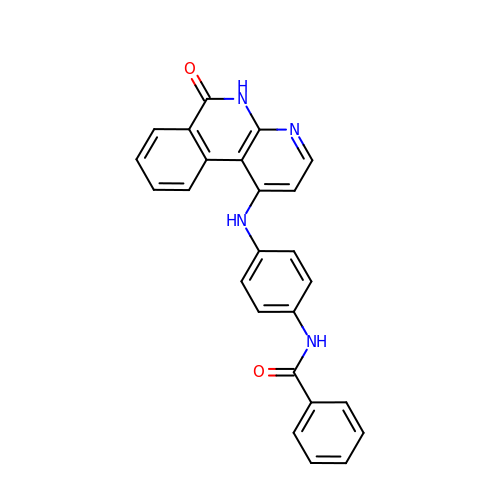N-{4-[(6-oxo-5,6-dihydrobenzo[c][1,8]naphthyridin-1-yl)amino]phenyl}benzamide | C25 H18 N4 O2 | XLSPYLMTRXPYKY-UHFFFAOYSA-N>MAHHHHHHFRIVVGLGKSGMSLVRYLARRGLPFAVVDTRENPPELATLRAQYPQVEVRCGELDAEFLCSARELYVSPGLSLRTPALVQAAAKGVRISGDIDLFAREAKAPIVAITGSNAKSTVTTLVGEMAVAADKRVAVGGNLGTPALDLLADDIELYVLELSSFQLETCDRLNAEVATVLNVSEDHMDRYDGMADYHLAKHRIFRGARQVVVNRADALTRPLIADTVPCWSFGLNKPDFKAFGLIEEDGQKWLAFQF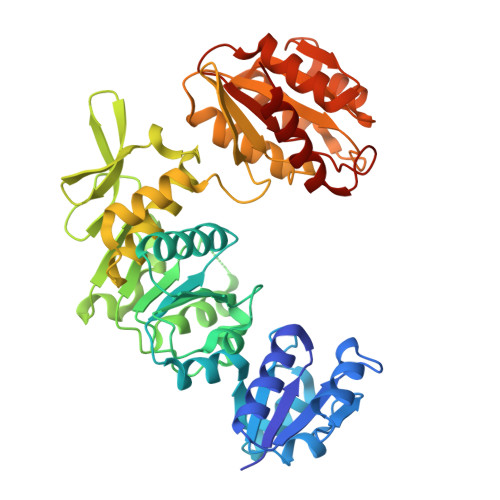DKLLPVGELKIRGAHNYSNALAALALGHAVGLPFDAMLGALKAFSGLAHRCQWVRERQGVSYYDDSKATNVGAALAAIEGLGADIDGKLVLLAGGDGKGADFHDLREPVARFCRAVVLLGRDAGLIAQALGNAVPLVRVATLDEAVRQAAELAREGDAVLLSPACASLDMFKNFEERGRLFAKAVEELA[2x]>[2x]MRQIAIYGKGGIGKSTTTQNLTAALSTMGNNILLVGCDPKADSTRMLLGGLNQKTVLDTLRSEGDEGIDLDTVLQPGFGGIKCVESGGPEPGVGCAGRGIITSIGLLENLGAYTDDLDYVFYDVLGDVVCGGFAMPIREGKAKEIYIVASGELMAIYAAN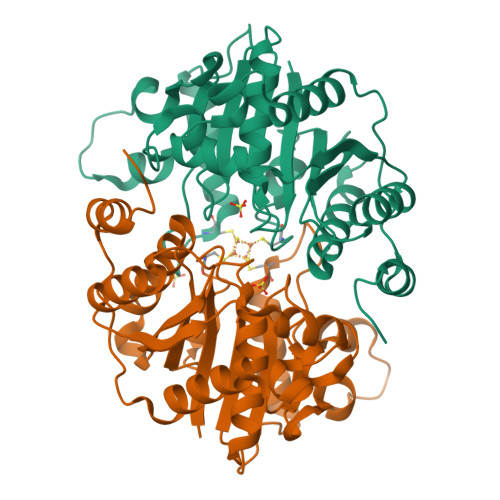NICKGLAKFAKGGARLGGIICNSRKVDGERELLEAFAKKLGSHLIHFVPRDNIVQRAEINRKTVIDFDRESDQAKEYLTLADNVQNNNKLVVPTPLPMEELEAMMVEFGIVEL diethyl 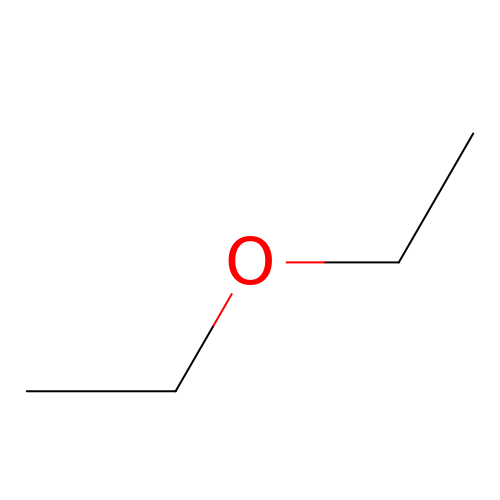ether | C4 H10 O | RTZKZFJDLAIYFH-UHFFFAOYSA-N>[2x]GSHMELEDSTLRYLQDLLAWVEENQHRVDGAEWGVDLPSVEAQLGSHRGLHQSIEEFRAKIERARSDEGQLSPATRGAYRDCLGRLDLQYAKLLNSSKARLRSLESLHSFVAAATK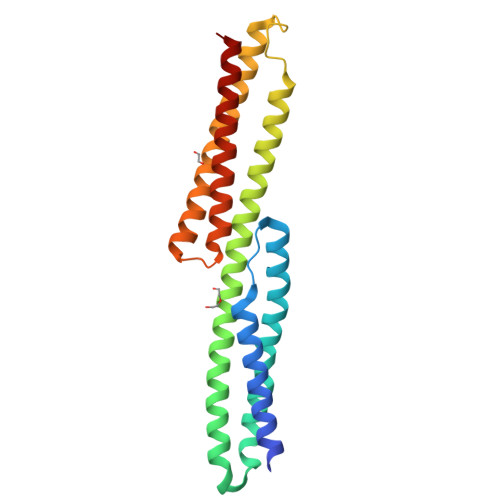ELMWLNEKEEEEVGFDWSDRNTNMTAKKESYSALMRELELKEKKIKELQNAGDRLLREDHPARPTVESFQAALQTQWSWMLQLCCCIEAHLKEN>MGHHHHHHGSMAKNTITKTLKLRIVRPYNSAEVEKIVADEKNNREKIALEKNKDKVKEACSKHLKVAAYCTT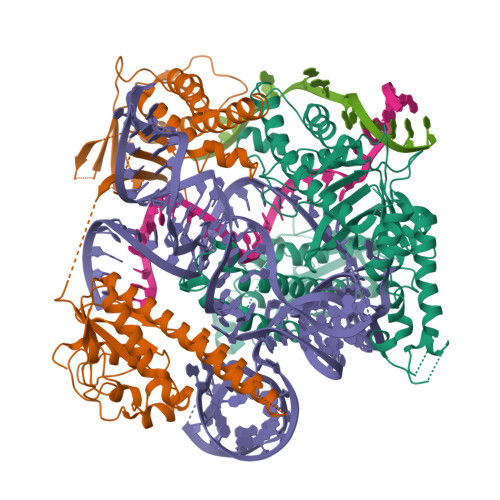QVERNACLFCKARKLDDKFYQKLRGQFPDAVFWQEISEIFRQLQKQAAEIYNQSLIELYYEIFIKGKGIANASSVEHYLSDVCYTRAAELFKNAAIASGLRSKIKSNFRLKELKNMKSGLPTTKSDNFPIPLVKQKGGQYTGFEISNHNSDFIIKIPFGRWQVKKEIDKYRPWEKFDFEQVQKSPKPISLLLSTQRRKRNKGWSKDEGTEAEIKKVMNGDYQTSYIEVKRGSKIGEKSAWMLNLSIDVPKIDKGVDPSIIGGIAVGVKSPLVCAINNAFSRYSISDNDLFHFNKKMFARRRILLKKNRHKRAGHGAKNKLKPITILTEKSERFRKKLIERWACEIADFFIKNKVGTVQMENLESMKRKEDSYFNIRLRGFWPYAEMQNKIEFKLKQYGIEIRKVAPNNTSKTCSKCGHLNNYFNFEYRKKNKFPHFKCEKCNFKENADYNAALNISNPKLKSTKEEP[2x]> MVAKGRIIRVTGPLVVADGMKGAKMYEVVRVGELGLIGEIIRLEGDKAVIQVYEETAGVRPGEPVVGTGASLSVELGPGLLTSIYDGIQRPLEVIREKTGDFIARGVTAPALPRDKKWHFIPKAKVGDKVVGGDIIGEVPETSIIVHKIMVPPGIEGEIVEIAEEGDYTIEEVIAKVKTPSGEIKELKMYQRWPVRVKRPYKEKLPPEVPLITGQRVIDTFFPQAKGGTAAIPGPFGSGKTVTQHQLAKWSDAQVVIYIGCGERGNEMTDVLEEFPKLKDPKTGKPLMERTVLIANTSNMPVAAREASIYTGITIAEYFRDMGYDVALMADSTSRWAEALREISGRLEEMPGEEGYPAYLASKLAEFYERAGRVVTLGSDYRVGSVSVIGAVSPPGGDFSEPVVQNTLRVVKVFWALDADLARRRHFPAINWLTSYSLYVDAVKDWWHKNIDPEWKAMRDKAMALLQKESELQEIVRIVGPDALPERERAILLVARMLREDYLQQDAFDEVDTYCPPE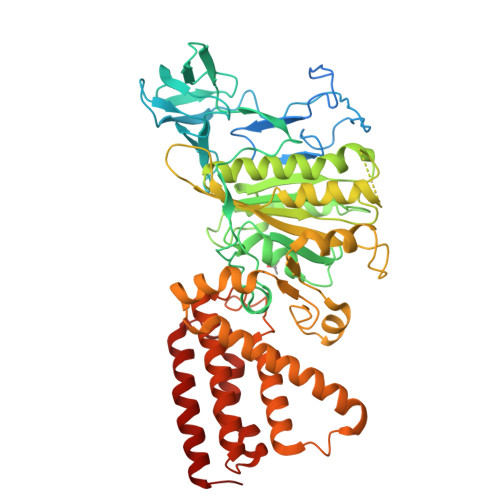KQVTMMRVLLNFYDKTMEAINRGVPLEEIAKLPVREEIGRMKFERDVSKIRSLIDKTNEQFEELFKKYGA>MAQK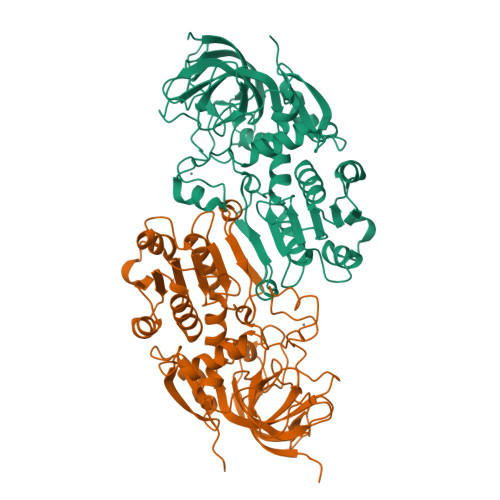APGVITCKAAVVWESSGPVVLEEIRVDPPKASEVRIKMLCASLCHTDVLCTKGFPIPLFPRIPGHEGVGVIESIGKDAKGLKPGDIVMPLYLGECGQCLNCKTGKTNLCHVYPPSFSGLMNDGTSRMSIARTGESIYHFASCSTWTEYAVADCNYVLKINPKISYPHASFLSCGFTTGFGATWRETQVSKGSSVAVFGIGTVGLGVIKGAQLQGASKIIGVDVNQYKAAKGKVFGMTDFINPKDHPDKSVSELVKELTHGLGVDHCFECTGVPSLLNEALEASKIGIGTVVPIGAGGEASVAINSLILFSGRTLKFTAFGGVRTQSDLPVIIDKCLNKEIQLDELLTHEIHLDNIQEAFEILKKPDCVKILIKFLEHHHHHH[4x]1-HYDROXY-2-S-GLUTATHIONYL-3-PARA-NITROPHENOXY-PROPANE | C19 H26 N4 O10 S | 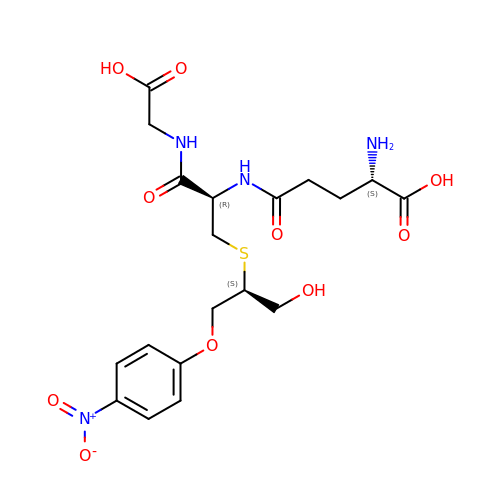YWXHXYSGHBAIBL-KKUMJFAQSA-N> SNAASTQYMELNQRDEKSPFRNANLRKAISYSIDRKALVESILGDGSIEPNGLVPADMAKDPSGGKDFAKEAGSQIEYDTKKAKEYWEKAKKELGISTLTMDILSSDADSSKKTVEFVQGSIQDALDGVKVTVSPVPFSVRLDRSNKGDFD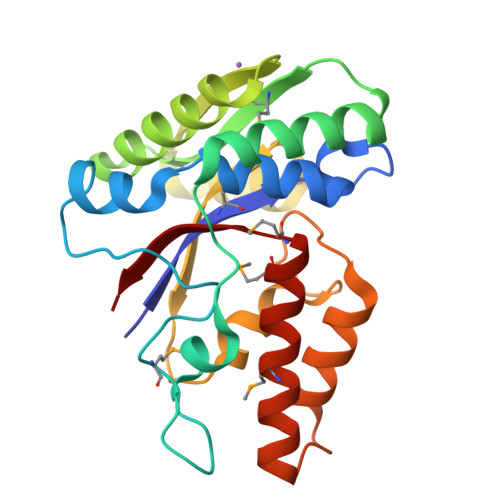AVIGGWSADYADPSSFLDLFASDNSYNRGRYNNAEFDKFVKAASSADATDPEKRWDDMLNAEKTIMGDMGVVPLFQKS> MHHHHHHMIEWIIRRSVANRFLVLMGALFLSIWGTWTIINTPVDALPDLSDVQVIIKTSYPGQAPQIVENQVTYPLTTTMLSVPGAKTVRGFSQFGDSYVYVIFEDGTDPYWARSRVLEYLNQVQGKLPAGVSAELGPDATGVGWIYEYALVDRSGKHDLADLRSLQDWFLKYELKTIPDVAEVASVGGVVKEYQVVIDPQRLAQYGISLAEVKSALDASNQEAGGSSIELAEAEYMVRASGYLQTLDDFNHIVLKASENGVPVYLRDVAKVQIGPEMRRGIAELNGEGEVAGGVVILRSGKNAREVIAAVKDKLETLKSSLPEGVEIVTTYDRSQLIDRAIDNLSGKLLEEFIVVAVVCALFLWHVRSALVAIISLPLGLCIAFIVMHFQGLNANIMSLGGIAIAVGAMVAAAIVMIENAHKRLEEWQHQHPDATLDNKTRWQVITDASVEVGPALFISLLIITLSFIPIFTLEGQEGRLFGPLAFTKTYAMAGAALLAIVVIPILMGYWIRGKIPPESSNPLNRFLIRVYHPLLLKVLHWPKTTLLVAALSVLTVLWPLNKVGGEFLPQINEGDLLYMPSTLPGISAAEAASMLQKTDKLIMSVPEVARVFGKTGKAETATDSAPLEMVETTIQLKPQEQWRPGMTMDKIIEELDNTVRLPGLANLWVPPIRNRIDMLSTGIKSPIGIKVSGTVLADIDAMAEQIEEVARTVPGVASALAERLEGGRYINVEINREKAARYGMTVADVQLFVTSAVGGAMVGETVEGIARYPINLRYPQSWRDSPQALRQLPILTPMKQQITLADVADIKVSTGPSMLKTENARPTSWIYIDARDRDMVSVVHDLQKAIAEKVQLKPGTSVAFSGQFELLERANHKLKLMVPMTLMIIFVLLYLAFRRVGEALLIISSVPFALVGGIWLLWWMGFHLSVATGTGFIALAGVAAEFGVVMLMYLRHAIEAVPSLNNPQTFSEQKLDEALYHGAVLRVRPKAMTVAVIIAGLLPILWGTGAGSEVMSRIAAPMIGGMITAPLLSLFIIPAAYKLMWLHRHRV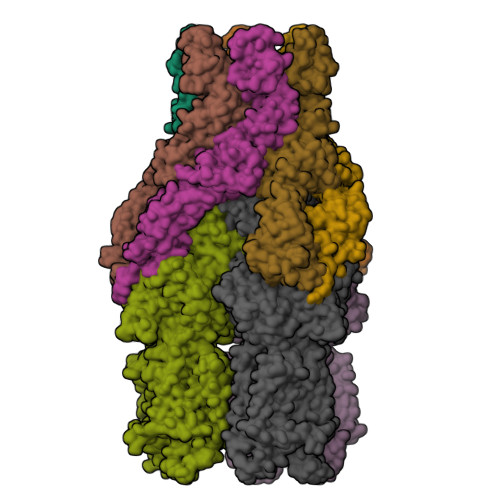RK;>MKKIALIIGSMIAGGIISAAGFTWVAKAEPPAEKTSTAERKILFWYDPMYPNTRFDKPGKSPFMDMDLVPKYADEESSASGVRIDPTQTQNLGVKTATVTRGPLTFAQSFPANVSYNEYQYAIVQARAAGFIDKVYPLTVGDKVQKGTPLLDLTIPDWVEAQSEYLLLRETGGTATQTEGILERLRLAGMPEADIRRLIATQKIQTRFTLKAPIDGVITAFDLRAGMNIAKDNVVAKIQGMDPVWVTAAIPESIAWLVKDASQFTLTVPARPDKTLTIRKWTLLPGVDAATRTLQLRLEVDNADEALKPGMNAWLQLNTASEPMLLIPSQALIDTGSEQRVITVDADGRFVPKRVAVFQASQGVTALRSGLAEGEKVVSSGLFLIDSEANISGALERMRSESATHAHHHHHHH[2x]>[2x]GHMVNMVSNPGFEDGLDSWQDWQQDMSAVPEAAHNGALGLKIGGGKAAGGGQDIPLKPNTTYILGAWAKFDSKPAGTF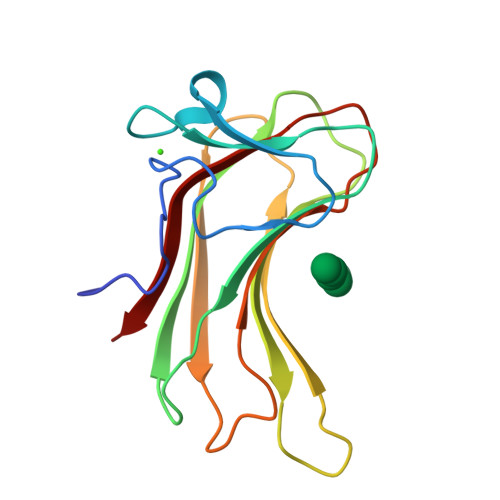DVVVQYHLKDANNTYVQHILNFNETDWTYKQLLFTTPDVFGSTPQLALWKGDTSKANLYVDDVYLVEV>[2x]GASKLRAVLEKLKLSRDDISTAAGMVKGVVDHLLLRLKCDSAFRGVGLLNTGSYYEHVKISAPNEFDVMFKLEVPRIQLEEYSNTRAYYFVKFKRNPKENPLSQFLEGEILSASKMLSKFRKIIKEEINDIKDTDVIMKRKRGGSPAVTLLISEKISVDITLALESKSSWPASTQEGLRIQNWLSAKVRKQLRLKPFYLVPKHAKEGNGFQEETWRLSFSHIEKEILNNHGKSK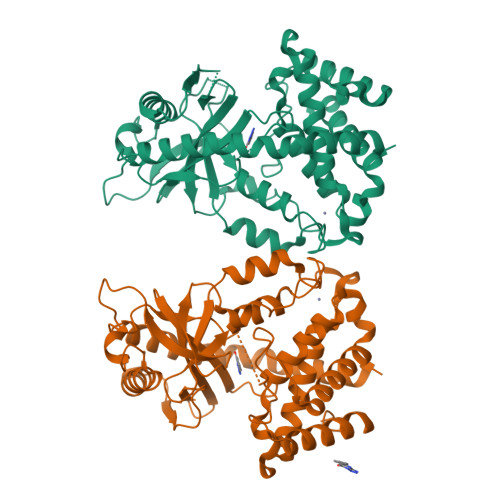TCCENKEEKCCRKDCLKLMKYLLEQLKERFKDKKHLDKFSSYHVKTAFFHVCTQNPQDSQWDRKDLGLCFDNCVTYFLQCLRTEKLENYFIPEFNLFSSNLIDKRSKEFLTKQIEYERNNEFPVFDEF>QFTDSCLRCICKVEGCDSQIGKCGMDVGSLSCGPYQIKKPYWIDCGKPGGGYESCTKNKACSETCVRAYMKRYGTFCTGGRT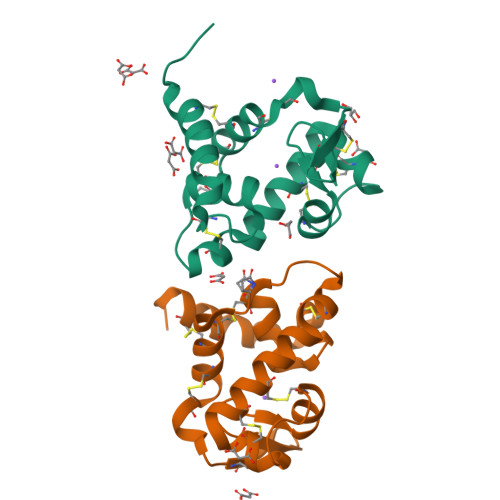PTCQDYARIHNGGPRGCKSSATVGYWNKVQKCLRGTHHHHHH[2x]5-fluoro-N-{4-[1-(2-hydroxy-2-methylpropanoyl)piperidin-4-yl]phenyl}-2H-isoindole-2-carboxamide | C24 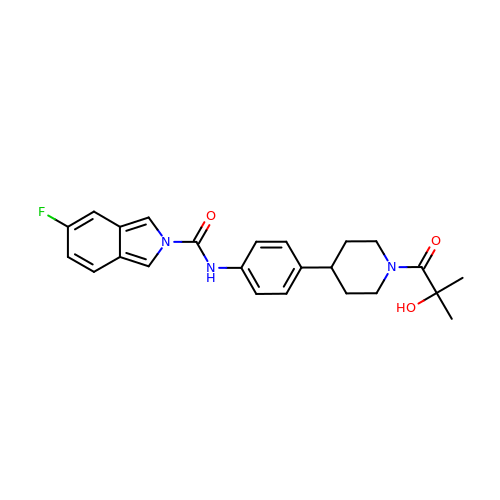H26 F N3 O3 | XZCZXZPDNUPSAB-UHFFFAOYSA-N>SGGGMLTLIQGKKIVNHLRSRLAFEYNGQLIKILSKNIVAVGSLRREEKMLNDVNLLIIVPEKKLLKHVLPNIRIKGLSFSVKVCGERKCVLFIEWEKKTYQLDLFTALAEEKPYAIFHFTGPVSYLIRIRAALKKKNYKLNQYGLFKNQT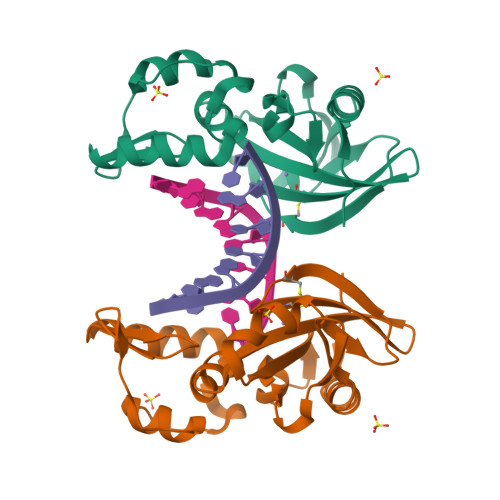LVPLKITTEKELIKELGFTYRIPKKRL[2x]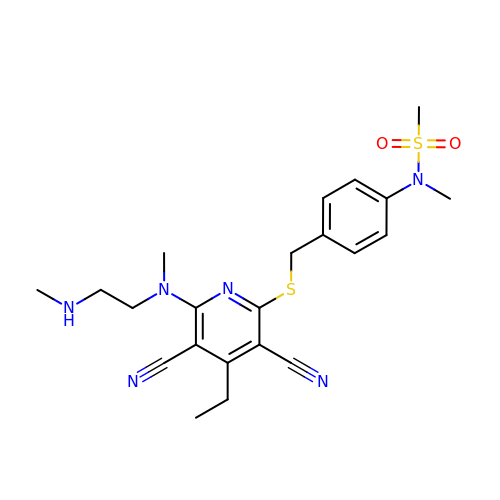N-(4-{[(3,5-dicyano-4-ethyl-6-{methyl[2-(methylamino)ethyl]amino}pyridin-2-yl)sulfanyl]methyl}phenyl)-N-methylmethanesulfonamide | C22 H28 N6 O2 S2 | GQHBHKILJGTNGL-UHFFFAOYSA-N> SMGKLSEHLRYCDSILREMLSKKHAAYAWPFYKPVDAEALELHDYHDIIKHPMDLSTVKRKMDGREYPDAQGFAADVRLMFSNCYKY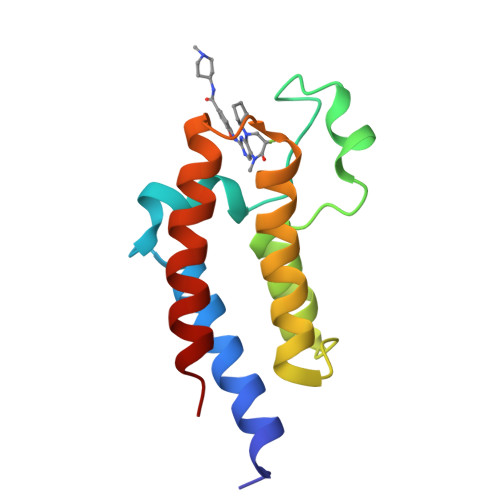NPPDHEVVAMARKLQDVFEMRFAKMP> MHHHHHHHAVRASEISRVYEAYPEKKATLYFLVLGFLALIVGSLFGPFQALNYGNVDAYPLLKRLLPFVQSYYQGLTLHGVLNAIVFTQLFAQAIMVYLPARELNMRPNMGLMWLSWWMAFIGLVVFALPLLANEATVLYTFYPPLKGHWAFYLGASVFVLSTWVSIYIVLDLWRRWKAANPGKVTPLVTYMAVVFWLMWFLASLGLVLEAVLFLLPWSFGLVEGVDPLVARTLFWWTGHPIMYFWLLPAYAIIYTILPKQAGGKLVSDPMARLAFLLFLLLSTPVGFHHQFADPGIDPTWKMIHSVLTL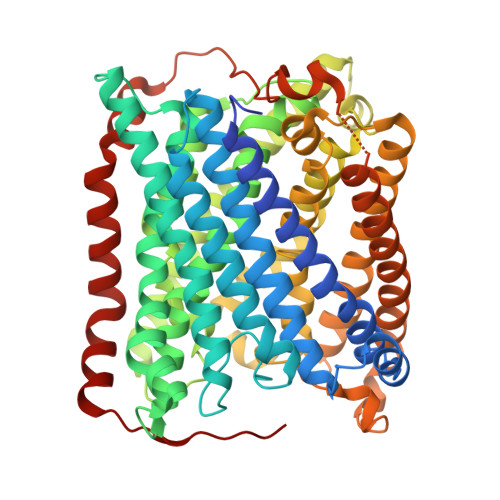FVAVPSLMTAFTVAASLEFAGRLRGGRGLFGWIRALPWDNPAFVAPVLGLLGFIPGGAGGIVNASFTLDYVVHNTAWVPGHFHLQVASLVTLTAMGSLYWLLPNLTGKPISDAQRRLGLAVVWLWFLGMMIMAVGLHWAGLLNVPRRAYIAQVPDAYPHAAVPMVFNVLAGIVLLVALLLFIYGLFSVLLSRERKPELAEAPLPFAEVISGPEDRRLVLAMDRIGFWFAVAAILVVLAYGPTLVQLFGHLNPVPGWRLW> KRPWKCCDEAVCTRSI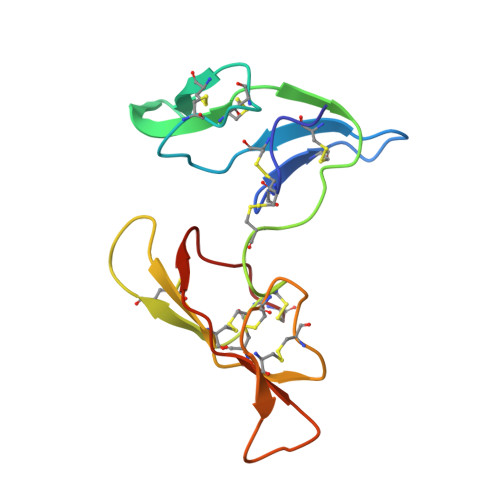PPICTCMDEVFECPKTCKSCGPSMGDPSRRICQDQYVGDPGPICRPWECCDKAICTRSNPPTCRCVDEVKKCAPTCKTCLPSRSRPSRRVCIDSYFGPVPPRCT>MVMMKLFYKPGACSLSPHIVLREAGLDFSIERVDLVTKKTETGADYLSINPKGQVPALVLDDGSLLTEGVAIVQYLADKVPDRHLIAPSGTLSRYHAIEWLNFIATELHKGFSPLFNPNTPDEYKTIVRERLDKQFSYVDSVLAEHDYLLG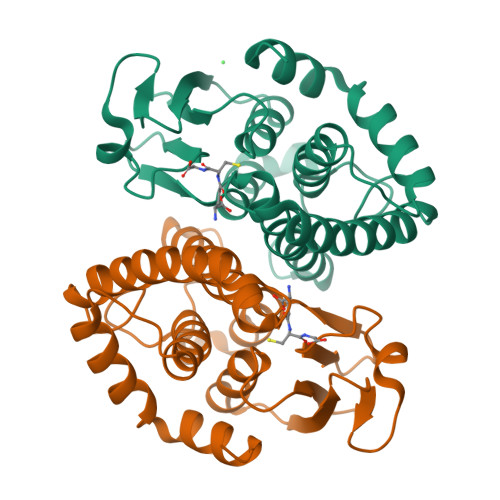KKFSVADAYLFTVSRWANALNLQIKERSHLDQYMARVAERPAVKAALAAEDIKAENLYFQ[2x]>MASVNPEYFSAADVYVPDEWEVAREKITMSRELGQGSFGMVYEGVAKGVVKDEPETRVAIKTVNEAASMRERIEFLNEASVMKEFNCHHVVRLLGVVSQGQPTLVIMELMTRGDLKSYLRSLRPEMENNPVLAPPSLSKMIQMAGEIADGMAYLNANKFVHRDLAARNCMVAEDFTVKIGDFGMTRDIYETDYYRKGGKGLLPVRWMSPESLKDGVFTTYSDVWSFGVVLWEIATLAEQPYQGLSNEQVLRFVMEGGLLDKPDNCPDMLFELMRMCWQYNP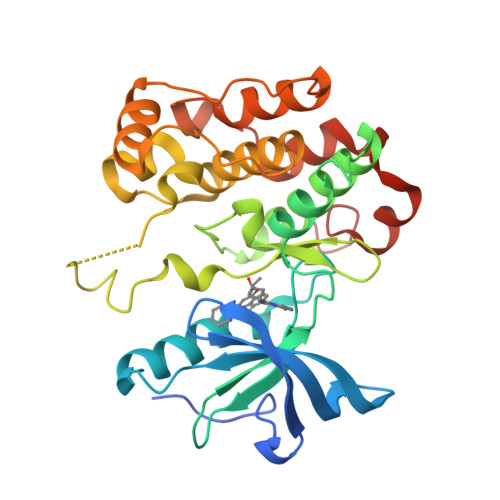KMRPSFLEIISSIKEEMEPGFREVSFYYSEENKAENLYFQ[8x]> PSRVVYLGSIPYDQTEEQILDLCSNVGPVINLKMMFDPQTGRS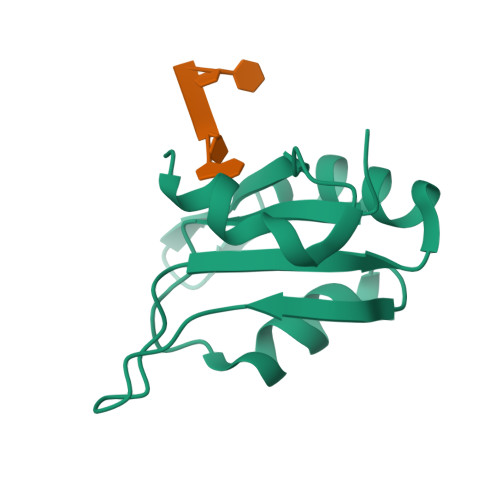KGYAFIEFRDLESSASAVRNLNGYQLGSRFLKCGYSSNSDISGVSLEHHHHHH Drosophila PGRP-LB belongs to the amidase PGRPs and downregulates the immune deficiency (IMD) pathway by cleaving meso-2,6-diaminopimelic (meso-DAP or DAP)-type PGN. The structure of the PGRP domain comprises three α-helices and one central β-sheet composed of six β-strands, similar to the bacteriophage T7 lysozyme, a zinc-dependent amidase. The main difference between amidase and non-catalytic PGRPs is the presence of Zn2+ in only amidase PGRPs, which is coordinated by two histidines and one cysteine. We generated mutants to characterize the amidase reaction mechanism and solved the X-ray structures of wild-type Drosophila PGRP-LBPA/PC and its mutants in apo form or complexed to TCT.

Our results show, however, that the activity of the H42A, H152A and C160S PGRP-LBPA/PC mutants depends on the substrate type and is either significantly reduced or completely abolished. Y78F and C160S PGRP-LBPA/PC mutant structures were elucidated to 1.30 Å and 1.40 Å resolution, respectively. Both mutants Y78F and C160S PGRP-LBPA/PC share a similar fold with PGRP-LBPA/PC wild type with a RMSD on Cα of 0.49 Å and 1.12 Å, respectively, but in different space groups, P6122 for PGRP-LBPA/PC_Y78F and P1 for PGRP-LBPA/PC_C160S. However, major structural changes were observed in PGRP-LBPA/PC_C160S structure around the mutation. The loop between the β6 sheet and the α3 helix is drifting apart from the active site with a RMSD of 2.37 Å, calculated on the Cα from the residues 148 to 172. This deviation is due to the loss of interaction between C160 and Zn2+, where the cysteine is replaced by a serine. We showed that Zn2+ is totally absent in PGRP-LBPA/PC_C160S mutant as already observed in the structure resolution, while it is still present in PGRP-LBPA/PC_Y78A mutant and PGRP-LBPA/PC wild type. Finally, the addition of Zn2+ to the reaction buffer used for activity assays allowed a small residual amidase activity of PGRP-LBPA/PC_C160S, whereas the absence of Zn2+ in the buffer totally abolished the amidase activity of PGRP-LBPA/PC_C160S, which is consistent with X-ray structural data. These data suggest that the C160 residue is needed to retain Zn2+ in the active site but not essential for residual amidase activity if Zn2+ is present in the media.

>GPMQQANLGDGVATARLLSRSDWGARLPKSVEHFQGPAPYVIIHHSYMPAVCYSTPDCMKSMRDMQDFHQLERGWNDIGYSFGIGGDGMIYTGRGFNVIGAHAPKYNDKSVGIVLIGDWRTELPPKQMLDAAKNLIAFGVFKGYIDPAYKLLGHRQVRDTESPGGRLFAEISSWPHFTHINDTEGVSSTTAPVVPHVHPQAAAPQKPHQSPPAAPKV[2x]>[2x]PDKENKKLLCRKCKALACYTADVRVIEECHYTVLGDAFKECFVSRPHPKPKQFSSFEKRAKIFCARQNCSHDWGIHVKYKTFEIP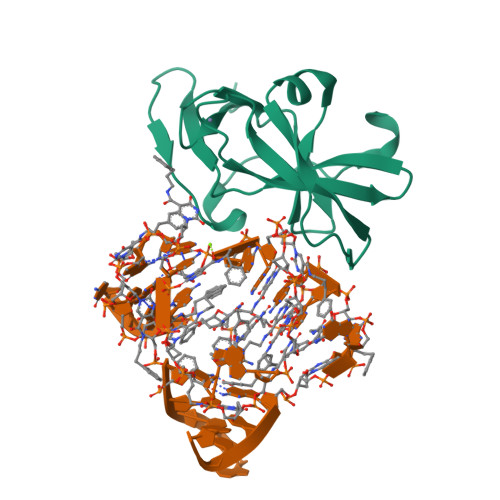VIKIESFVVEDIATGVQTLYSKWKDFHFEKIPFDPAEMSK>MAAAMASAELQGKYQKLAQEYSKLRAQNQVLKKGVVDEQANSAALKEQLKMKDQSLRKLQQEMDSLTFRNLQLAKRVELLQDELALSEPRGKKNKKSGESSSQLSQEQKSVFDEDLQKKIEENERLHIQFFEADEQHKHVEAELRSRLATLETEAAQHQAVVDGLTRKYMETIEKLQNDKAKLEVKSQTLEKEAKECRLRTEECQLQLKTLHEDLSGRLEESLSIINEKVPFNDTKYSQYNALNVPLHNRRHQLKMRDIAGQALAFVQDLVTALLNFHTYTEQRIQIFPVDSAIDTISPLNQKFSQYLHENASYVRPLEEGMLHLFESITEDTVTVLETTVKLKTFSEHLTSYICFLRKILPYQLKSLEEECESSLCTSALRARNLELSQDMKKMTAVFEKLQTYIALLALPSTEPDGLLRTNYSSVLTNVGAALHGFHDVMKDISKHYSQKAAIEHELPTATQKLITTNDCILSSVVALTNGAGKIASFFSNNLDYFIASLSYGPKAASGFISPLSAECMLQYKKKAAAYMKSLRKPLLESVPYEEALANRRILLSSTESREGLAQQVQQSLEKISKLEQEKEHWMLEAQLAKIKLEKENQRIADKLKNTGSAQLVGLAQENAAVSNTAGQDEATAKAVLEPIQSTSLIGTLTRTSDSEVPDVESREDLIKNHYMARIVELTSQLQLADSKSVHFYAECRALSKRLALAEKSKEALTEEMKLASQNISRLQDELTTTKRSYEDQLSMMSDHLCSMNETLSKQREEIDTLKMSSKGNSKKNKSR[2x];>[2x]MSHHHHHHKGLYFQQSSTDEEITFVFQEKEDLPVTEDNFVKLQVKACALSQINTKLLAEMKMKKDLFPVGREIAGIVLDVGSKVSFFQPDDE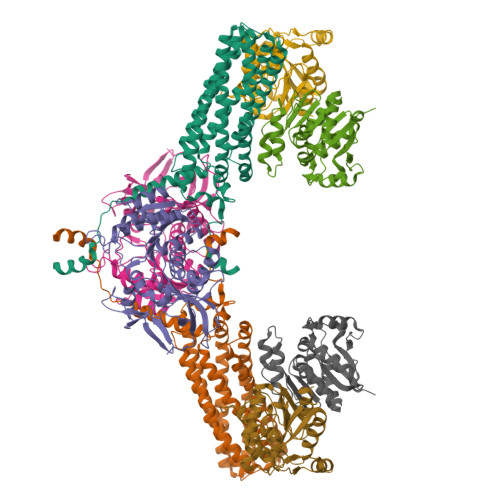VVGILPLDSEDPGLCEVVRVHEHYLVHKPEKVTWTEAAGSIRDGVRAYTALHYLSHLSPGKSVLIMDGASAFGTIAIQLAHHRGAKVISTACSLEDKQCLERFRPPIARVIDVSNGKVHVAESCLEETGGLGVDIVLDAGVRLYSKDDEPAVKLQLLPHKHDIITLLGVGGHWVTTEENLQLDPPDSHCLFLKGATLAFLNDEVWNLSNVQQGKYLCILKDVMEKLSTGVFRPQLDEPIPLYEAKVSMEAVQKNQGRKKQVVQF;>MSHHHHHHASERLPNRPACLLVASGAAEGVSAQSFLHCFTMASTAFNLQVATPGGKAMEFVDVTESNARWVQDFRLKAYASPAKLESIDGARYHALLIPSCPGALTDLASSGSLARILQHFHSESKPICAVGHGVAALCCATNEDRSWVFDSYSLTGPSVCELVRAPGFARLPLVVEDFVKDSGACFSASEPDAVHVVLDRHLVTGQNASSTVPAVQNLLFLCGSRK[4x]>[4x]ATQGVFTLP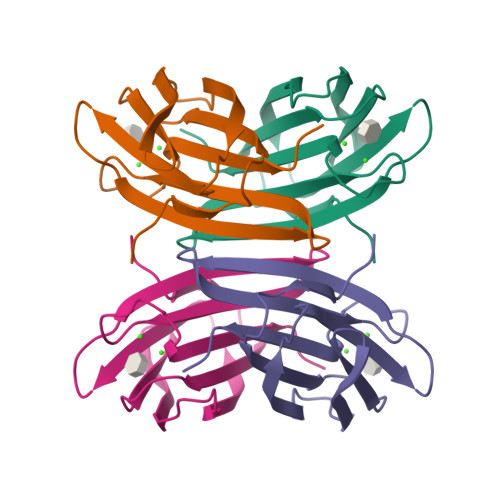ANTQFGVTAFANSAGTQTVNVQVNNETVATFTGQSTNNAIIGSKVLNSGGGGKVQILVSVNGRSSDLVSAQVILANELNFALVGSEDSTDNDYNDAVVVINWPLG> MMFGRFTERAQKVLALAQEEALRLGHNNIGTEHILLGLVREGEGIAAKALQALGLGSEKIQKEVESLIGRGQEMSQTIHYTPRAKKVIELSMDEARKLGHSYVGTEHILLG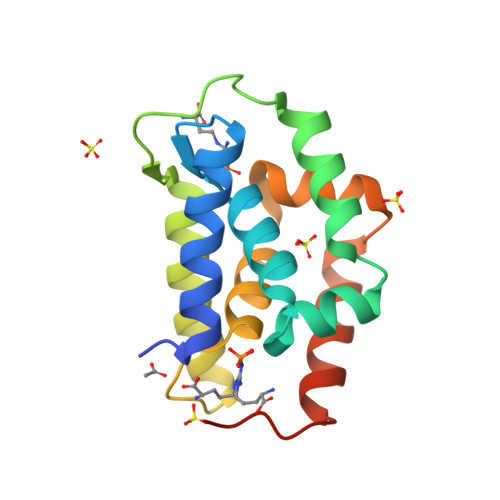LIREGEGVAARVLNNLGVSLNKARQQVLQLLGSNETGSSHHHHHH>[10x]ASGNARIGKPAPDFKATAVVDGAFKEVKLSDYKGKYVVLFFYPLDFTFVCPTEIIAFSNRAEDFRKLGCEVLGVSVDSQFTHLAWINT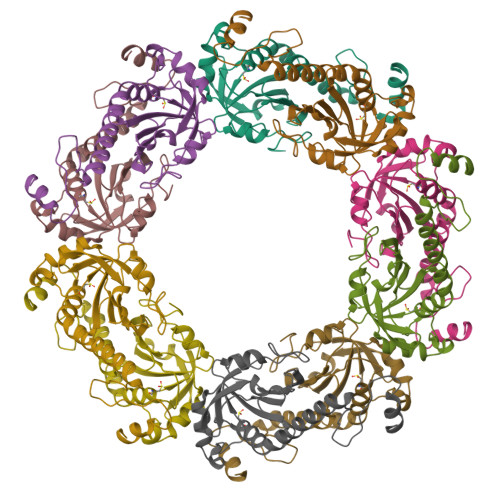PRKEGGLGPLNIPLLADVTRRLSEDYGVLKTDEGIAYRGLFIIDGKGVLRQITVNDLPVGRSVDEALRLVQAFQYTDEHGEVCPAGWKPGSDTIKPNVDDSKEYFSKHN P2X receptors are ATP-activated cation channels, and the P2X4 subtype plays important roles in the immune system and the central nervous system, particularly in neuropathic pain. Here, we report the cryo-EM structures of the zebrafish P2X4 receptor in complex with two P2X4 subtype-specific antagonists, BX430 and BAY-1797. Both antagonists bind to the same allosteric site located at the subunit interface at the top of the extracellular domain. The overall structures of the zebrafish P2X4 receptor in complex with BX430 and BAY-1797 are very similar and show a chalice-like trimeric architecture with each subunit containing a relatively large extracellular domain and two TM helices, resembling the shape of a dolphin, as in the previously reported P2X receptor structures.

BAY-1797, or N-[4-(3-chlorophenoxy)-3-sulfamoylphenyl]-2-phenylacetamide, is a sulfonamide antagonist of P2X4 with an IC50 of 211 nM and high subtype specificity. In our experiments, BAY-1797 inhibited ATP-dependent currents of both zfP2X4 and hP2X4 with comparable IC50 values of 0.14 µM and 0.24 µM, respectively. In the BAY-1797-bound structure, the phenylacetamide moiety faces the outer side of the receptor, while the chlorophenoxy moiety faces the inner side. The BAY-1797 binding site also consists primarily of hydrophobic residues, which are the same as those of the BX430 binding site. Furthermore, both Asp91 and Lys301 are similarly involved in BAY-1797 binding, despite the structural differences between BAY-1797 and BX430. The main chain carbonyl group of Asp91 forms a hydrogen bond with the amine in the phenylacetamide moiety of BAY-1797, and the hydrophobic part of the Lys301 side chain interacts with the phenyl group of the phenylacetamide moiety by forming a cation-pi interaction between the side chain of Lys301 and the aromatic ring of Tyr302. While most of the residues involved in BAY-1797 binding overlap with those involved in BX430 binding, there are also specific interactions in the binding of BAY-1797. The amine of the sulfonamide group forms hydrogen bonds with the main chain carbonyl groups of Ala90 and Ile93. Finally, the chlorophenoxy moiety of BAY-1797 protrudes into the center of the receptor and forms hydrophobic contacts with the corresponding portion of the other two BAY-1797 molecules in the trimer. From another perspective, while the configurations of BX430 and BAY-1797 in the zfP2X4 structure are very similar, BAY-1797 has bulkier functional groups deeper in the receptor that mediate the BAY-1797-specific interactions. Further close inspection of the allosteric site revealed that in the apo state, the side chain of Lys301 faces the inside of the receptor, which would cause steric hindrance with the pyridine group of BX430 in the BX430-bound structure.

>[3x]DSVSQCFFDYYTSKILIIRSKKVGTLNRFTQALVIAYVIGYVCVYNKGYQDTDTVLSSVTTKVKGIALTNTSELGERIWDVADYIIPPQEDGSFFVLTNMIITTNQTQSKCAENPTPASTCTSHRDCKRGFNDARGDGVRTGRCVSYSASVKTCEVLSWCPLEKIVDPPNPPLLADAENFTVLIKNNIRYPKFNFNKRNILPNINSSYLTHCVFSRKTDPDCPIFRLGDIVGEAEEDFQIMAVRGGVMGVQIRWDCDLDMPQSWCVPRYTFRRLDNKDPDNNVAPGYNFRFAKYYKNSDGTETRTLIKGYGIRFDVMVFGQAGKFNIIPTLLNIGAGLALLGLVNVICDW5-[2-amino-3-(1-methyl-1H-pyrazol-4-yl)pyrazolo[1,5-a]pyrimidin-5-yl]-2-[(1S)-1-cyclopropylethyl]-7-(trifluoromethyl)-2,3-dihydro-1H-isoindol-1-one | C24 H22 F3 N7 O | 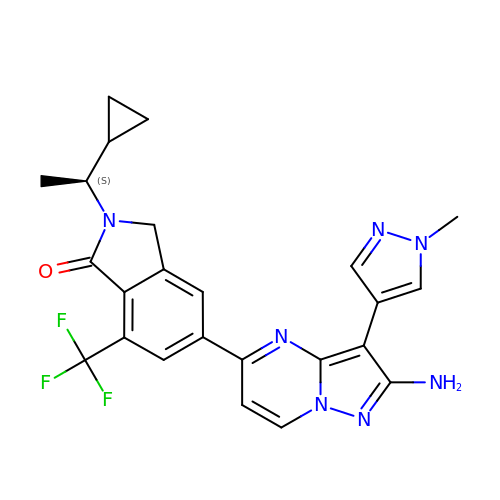CYAPSTHKVSVUQB-LBPRGKRZSA-N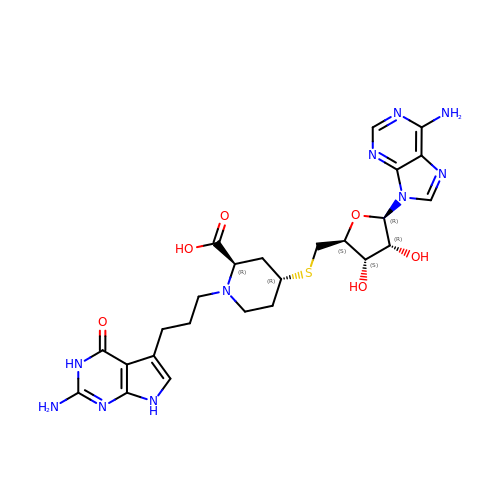5'-S-{(2R,4R)-1-[3-(2-amino-4-oxo-4,7-dihydro-3H-pyrrolo[2,3-d]pyrimidin-5-yl)propyl]-2-carboxypiperidin-4-yl}-5'-thioadenosine | C25 H32 N10 O6 S | AOZGSZXCWJDLPF-LVEUASCASA-N>[2x]MKKTKIVCTIGPKTESEEMLAKMLDAGMNVMRLNFSHGDYAEHGQRIQNLRNVMSKTGKTA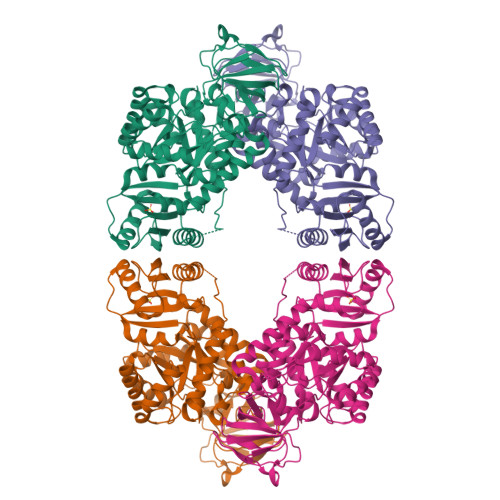AILLDTKGQEIRTMKLEGGNDVSLKAGQTFTFTTDKSVIGNSEMVAVTYEGFTTDLSVGNTVLVDDGLIGMEVTAIEGNKVICKVLNNGDLGENKGVNLPGVSIALPALAEKDKQDLIFGCEQGVDFVAASFIRKRSDVIEIREHLKAHGGENIHIISKIENQEGLNNFDEILEASDGIMVARGDLGVEIPVEEVIFAQKMMIEKCIRARKVVITATQMLDSMIKNPRPTRAEAGDVANAILDGTDAVMLSGESAKGKYPLEAVSIMATICERTDRVMNSRLEFNNDNRKLRITEAVCRGAVETAEKLDAPLIVVATQGGKSARAVRKYFPDATILALTTNEKTAHQLVLSKGVVPQLVKEITSTDDFYRLGKELALQSGLAHKGDVVVMVSGALVPSGTTNTASVHVL>[2x]TQPMIKKIMSRLFSAFDVTHLGYLTPDKVEEVCRYLGRNMSDGDVKAMKAEINAIDGHVTFEKFWAWWCSHPVHSRTKCFSMVSADFSMPYHQQQLVVHEKGEMYTPSYRVLYFFRDLETGRERQVSPWHDIPLYVRDLVRTKPEATPMNRYNFICEIPKWTRAKFEIATGESFNPIKQ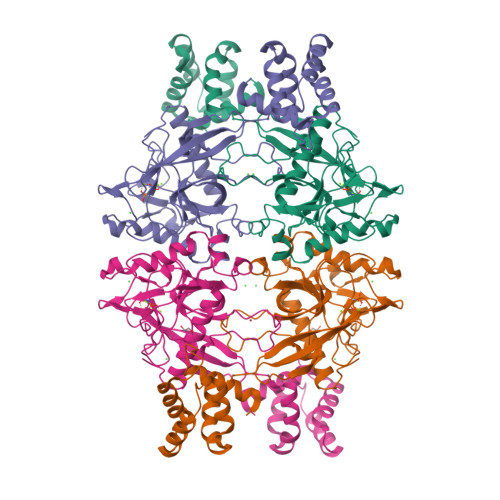DIKNGVPRFYKHGDMMWNYGAFPQTWESTEVLFEAGVTGDNDPVDAVEIGMTQFKVGQVSAVKVLGVLGMIDEGKMDWKVVCISHNDPICRFMKDIHDVPKFLPGCLDAIREWFRVYKICQGGEASHFAFDGEFKDKEYAMKVIDESHNMWHNLLKVNKRGEL> MSRRAPGSRLSSGGGGGGTKYPRSWNDWQPRTDSASADPDNLKYSSSRDRGGSSSYGLQPSNSAVVSRQRHDDTRVHADIQNDEKGGYSVNGGSGENTYGRKSLGQELRVNNVTSPEFTSVQHGSRALATKDMRKSQERSMSYSDESRLSNLLRRITREDDRDRRLATVKQLKEFIQQPENKLVLVKQLDNILAAVHDVLNESSKLLQELRQEGACCLGLLCASLSYEAEKIFKWIFSKFSSSAKDEVKLLYLCATYKALETVGEKKAFSSVMQLVMTSLQSILENVDTPELLCKCVKCILLVARCYPHIFSTNFRDTVDILVGWHIDHTQKPSLTQQVSGWLQSLEPFWVADLAFSTTLLGQFLEDMEAYAEDLSHVASGESVDEDVPPPSVSLPKLAALLRVFSTVVRSIGERFSPIRGPPITEAYVTDVLYRVMRCVTAANQVFFSEAVLTAANECVGVLLGSLDPSMTIHCDMVITYGLDQLENCQTCGTDYIISVLNLLTLIVEQINTKLPSSFVEKLFIPSSKLLFLRYHKEKEVVAVAHAVYQAVLSLKNIPVLETAYKLILGEMTCALNNLLHSLQLPEACSEIKHEAFKNHVFNVDNAKFVVIFDLSALTTIGNAKNSLIGMWALSPTVFALLSKNLMIVHSDLAVHFPAIQYAVLYTLYSHCTRHDHFISSSLSSSSPSLFDGAVISTVTTATKKHFSIILNLLGILLKKDNLNQDTRKLLMTWALEAAVLMKKSETYAPLFSLPSFHKFCKGLLANTLVEDVNICLQACSSLHALSSSLPDDLLQRCVDVCRVQLVHSGTRIRQAFGKLLKSIPLDVVLSNNNHTEIQEISLALRSHMSKAPSNTFHPQDFSDVISFILYGNSHRTGKDNWLERLFYSCQRLDKRDQSTIPRNLLKTDAVLWQWAIWEAAQFTVLSKLRTPLGRAQDTFQTIEGIIRSLAAHTLNPDQDVSQWTTADNDEGHGNNQLRLVLLLQYLENLEKLMYNAYEGCANALTSPPKVIRTFFYTNRQTCQDWLTRIRLSIMRVGLLAGQPAVTVRHGFDLLTEMKTTSLSQGNELEVTIMMVVEALCELHCPEAIQGIAVWSSSIVGKNLLWINSVAQQAEGRFEKASVEYQEHLCAMTGVDCCISSFDKSVLTLANAGRNSASPKHSLNGESRKTVLSKPTDSSPEVINYLGNKACECYISIADWAAVQEWQNAIHDLKKSTSSTSLNLKADFNYIKSLSSFESGKFVECTEQLELLPGENINLLAGGSKEKIDMKKLLPNMLSPDPRELQKSIEVQLLRSSVCLATALNPIEQDQKWQSITENVVKYLKQTSRIAIGPLRLSTLTVSQSLPVLSTLQLYCSSALENTVSNRLSTEDCLIPLFSEALRSCKQHDVRPWMQALRYTMYQNQLLEKIKEQTVPIRSHLMELGLTAAKFARKRGNVSLATRLLAQCSEVQLGKTTTAQDLVQHFKKLSTQGQVDEKWGPELDIEKTKLLYTAGQSTHAMEMLSSCAISFCKSVKAEYAVAKSILTLAKWIQAEWKEISGQLKQVYRAQHQQNFTGLSTLSKNILTLIELPSVNTMEEEYPRIESESTVHIGVGEPDFILGQLYHLSSVQAPEVAKSWAALASWAYRWGRKVVDNASQGEGVRLLPREKSEVQNLLPDTITEEEKERIYGILGQAVCRPAGIQDEDITLQITESEDNEEDDMVDVIWRQLISSCPWLSELDESATEGVIKVWRKVVDRIFSLYKLSCSAYFTFLKLNAGQIPLDEDDPRLHLSHRVEQSTDDMIVMATLRLLRLLVKHAGELRQYLEHGLETTPTAPWRGIIPQLFSRLNHPEVYVRQSICNLLCRVAQDSPHLILYPAIVGTISLSSESQASGNKFSTAIPTLLGNIQGEELLVSECEGGSPPASQDSNKDEPKSGLNEDQAMMQDCYSKIVDKLSSANPTMVLQVQMLVAELRRVTVLWDELWLGVLLQQHMYVLRRIQQLEDEVKRVQNNNTLRKEEKIAIMREKHTALMKPIVFALEHVRSITAAPAETPHEKWFQDNYGDAIENALEKLKTPLNPAKPGSSWIPFKEIMLSLQQRAQKRASYILRLEEISPWLAAMTNTEIALPGEVSARDTVTIHSVGGTITILPTKTKPKKLLFLGSDGKSYPYLFKGLEDLHLDERIMQFLSIVNTMFATINRQETPRFHARHYSVTPLGTRSGLIQWVDGATPLFGLYKRWQQREAALQAQKAQDSYQTPQNPGIVPRPSELYYSKIGPALKTVGLSLDVSRRDWPLHVMKAVLEELMEATPPNLLAKELWSSCTTPDEWWRVTQSYARSTAVMSMVGYIIGLGDRHLDNVLIDMTTGEVVHIDYNVCFEKGKSLRVPEKVPFRMTQNIETALGVTGVEGVFRLSCEQVLHIMRRGRETLLTLLEAFVYDPLVDWTAGGEAGFAGAVYGGGGQQAESKQSKREMEREITRSLFSSRVAEIKVNWFKNRDEMLVVLPKLDGSLDEYLSLQEQLTDVEKLQGKLLEEIEFLEGAEGVDHPSHTLQHRYSEHTQLQTQQRAVQEAIQVKLNEFEQWITHYQAAFNNLEATQLASLLQEISTQMDLGPPSYVPATAFLQNAGQAHLISQCEQLEGEVGALLQQRRSVLRGCLEQLHHYATVALQYPKAIFQKHRIEQWKTWMEELICNTTVERCQELYRKYEMQYAPQPPPTVCQFITATEMTLQRYAADINSRLIRQVERLKQEAVTVPVCEDQLKEIERCIKVFLHENGEEGSLSLASVIISALCTLTRRNLMMEGAASSAGEQLVDLTSRDGAWFLEELCSMSGNVTCLVQLLKQCHLVPQDLDIPNPMEASETVHLANGVYTSLQELNSNFRQIIFPEALRCLMKGEYTLESMLHELDGLIEQTTDGVPLQTLVESLQAYLRNAAMGLEEETHAHYIDVARLLHAQYGELIQPRNGSVDETPKMSAGQMLLVAFDGMFAQVETAFSLLVEKLNKMEIPIAWRKIDIIREARSTQVNFFDDDNHRQVLEEIFFLKRLQTIKEFFRLCGTFSKTLSGSSSLEDQNTVNGPVQIVNVKTLFRNSCFSEDQMAKPIKAFTADFVRQLLIGLPNQALGLTLCSFISALGVDIIAQVEAKDFGAESKVSVDDLCKKAVEHNIQIGKFS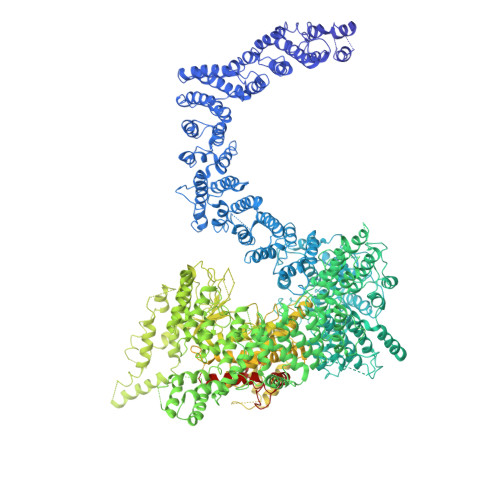QLVMNRATVLASSYDTAWKKHDLVRRLETSISSCKTSLQRVQLHIAMFQWQHEDLLINRPQAMSVTPPPRSAILTSMKKKLHTLSQIETSIATVQEKLAALESSIEQRLKWAGGANPALAPVLQDFEATIAERRNLVLKESQRASQVTFLCSNIIHFESLRTRTAEALNLDAALFELIKRCQQMCSFASQFNSSVSELELRLLQRVDTGLEHPIGSSEWLLSAHKQLTQDMSTQRAIQTEKEQQIETVCETIQNLVDNIKTVLTGHNRQLGDVKHLLKAMAKDEEAALADGEDVPYENSVRQFLGEYKSWQDNIQTVLFTLVQAMGQVRSQEHVEMLQEITPTLKELKTQSQSIYNNLVSFASPLVTDATNECSSPTSSATYQPSFAAAVRSNTGQKTQPDVMSQNARKLIQKNLATSADTPPSTVPGTGKSVACSPKKAVRDPKTGKAVQERNSYAVSVWKRVKAKLEGRDVDPNRRMSVAEQVDYVIKEATNLDNLAQLYEGWTAWV> GAMEADLSEPFSLTEVQTAYMLGRNPQFELSGISPQTYFEYETELDIARLSRSFQKVIQRHPMLRAVILPEGKQQILRDVPEYEIEVESLVSMPPEKQAARLREERSRMIDHVFPLGQWPLFELKAFQLQEHTYLLCFRYDALLMDGASMNLVGQDLMHYYHQPDAQLPPLSFTFQDYMHIYDDMKRGTEYETAKAYWTNKLPDFPPAPSLLLAKDPAEIGTPNFQSLTTIITKDKWLKLRRLAQDKQVTPSALLCTVYGEVLAFWSNQRRLAINLTVFNRYPVHDEVEQIVGDFTSLILLDMDMDQKQPFFTKVEQTQSTLLDGLEHRHYDGVEFIRDYTRYHQMRPKAVMPIVFTSMLAGAGAFAWEEIGSLRHIHARTPQVYLDNVVIEKNGELLVSWNYVEELFDAEVMESMFTQFVELLDQLVEQGDINPLRISQKDYALIDQYNATAEPIPAATLHQLFIDQAQRTPDQVAVVFEQEWLTYSELDQRSNQVARFLQSRGIGRGDRVGVLA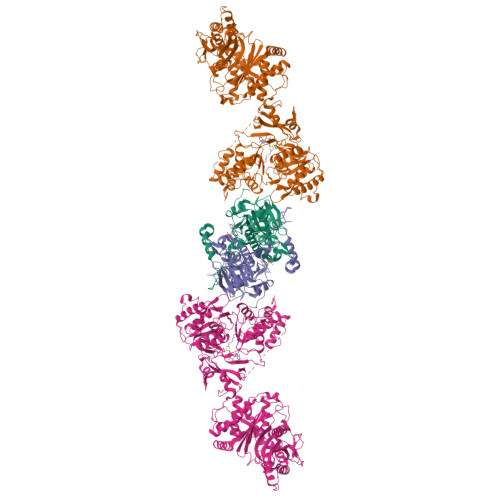KRQVETIINLMAVLKAGAAYVPIDPDHPYERQTYILENSSCKILLDSDLYETMEISSYADGDLTPVAEPEDTAYVIYTSGSTGRPKGVIITHQAASNTIQDINRKFEVNEEDRIIGISSMCFDLSVYDIFGTLSAGATLVMIRDPRDMRELVRTVERRGITIWNTVPAIMDLALDHVGSHFENISLRLVLLSGDWIPLPLPAKINRHFPVADVISLGGATEASIWSIYWPIEQVEANWKSIPYGKPLANQTYYVLNYDQKMCPVGVIGDLYIGGAGLAQGYLNDDQKTKDAFIMHPEFGPIYKTGDCGRMRPEGYIEFLGRQDYQVKIQGYRVELEEISHCLLTYPDVDQAVVIDQTDERGMKFLVGYVVAQQEIDEKALRKHLMEHLPEYMIPAHLVHLEQLPLTPNGKLDRKALPVPKKQRNAEKFVAPQAGLEKILASVWQEVLNVEQIGANDHFFALGGDSIKAIQVSARLFVQGYHLDTKSLFEFPVLRDVARTIKKLAAAENLFY;> GAMGEQIFYWSPAKHWRMSDEGVVIGESTYTGMILEWFPEFYFFAQTGVTINRLLERFSSGSEKEANEILELLIQDRVLVEGILPPREVFSPQEGLFVNPYSEQIRYSKEALDYYVSEQLNRTHAACRSTKIQLETSGALPDIIQKRRSCRRFDMKTPVSFATFSNLLSSLKQRKEDKILYNYASAGGLYPIDVFVYVKPRRVEGVKAGFYYFNPADHSLVLVNNIDQVIKDDHELINQDIFAQSAFSVYLVYNARASMPKYGAAGYFYACIEAGIITATLNMVAEDLNVGLCSIGHMNFEEIQTFLKLEDHQVILHAIEGGLKIDGAAAENLFY>XPPGPPGPPGPPGLKGHRGFTGLQGPPGPPGPPG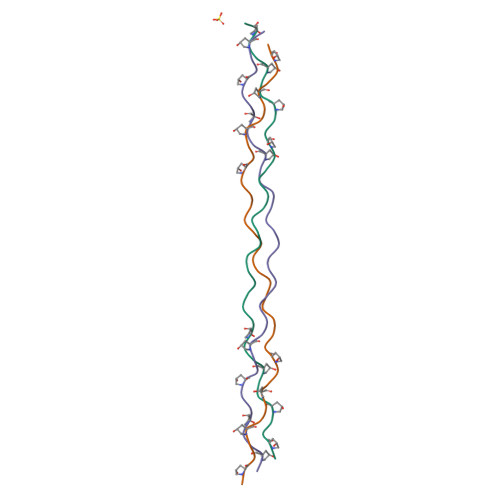PPGX[3x]> MAAPQPQAAAVSSASGVSGPGSAGGPGPQQQPQPTQLVGSAQSGLLQQQQQDFDPVQRYKMLIPQLKESLQTLMKVAAQNLIQNTNIDNGQKSSDAPLQRFDKCLEEFYALCDQLELCLRLAHECLSQSCDSAK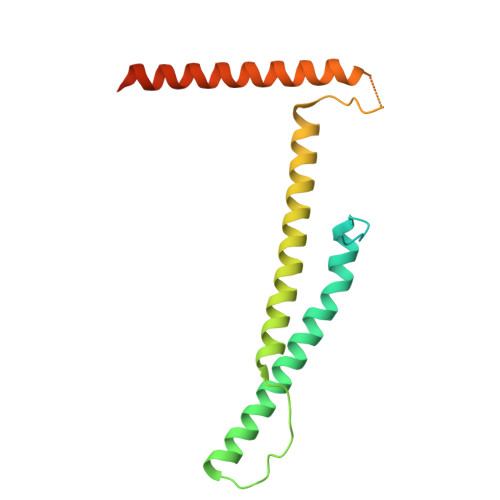HSPTLVPTATKPDAVQPDSLPYPQYLAVIKAQITCAKDIHTALLDCANKVTGKTTAPSTGPGGSL M1.HpyAVI is a DNA adenine MTase that belongs to the type II R-M system. M1.HpyAVI encoded by ORF hp0050 is an N6-adenine methyltransferase belonging to the β-class MTase. It has been reported recently that this enzyme recognizes the sequence of 5′-GAGG-3′, 5′-GGAG-3′ or 5′-GAAG-3′ and methylates adenines in these sequences. The structural basis and the catalytic mechanism underlying such a distinct activity are not well understood due to the lack of an available 3D structure of this enzyme.Here, we report the crystal structure of M1.HpyAVI from H. pylori 26695, which is the first determined N6-adenine MTase structure in H. pylori.

The cofactor-free and AdoMet-bound proteins were crystallized at different conditions. Both structures were determined by means of molecular replacement, and refined to 3.0 Å and 3.1 Å, respectively. Four and eight protein monomers resided in the asymmetric units of the two crystal structures. The two structures are very similar to each other and could be well overlaid with an RMSD of 0.76 Å on 191 Cα atoms. The catalytic motif DPPY lies in a loop connecting αD and β4, and the cofactor AdoMet binds in a neighboring cavity. The cofactor binding pocket of M1.HpyAVI is surrounded by residues 7-9, 29-31, 165-167, 216-218 and 221, which are conserved among most of DNA MTases. A hydrogen bond between D29 in the catalytic motif DPPY and the amino group of bound AdoMet is preserved as other MTase structures. Residues D8 and A9 from hydrogen-bonds with N6 and N1 of the purine ring, respectively, and E216 also locates at hydrogen bonding distance with O2′ and O3′ of the ribose. In addition, H168, T200 and S198 contact the terminal carboxyl of AdoMet. The phenyl ring of F195 forms a perpendicular π-stacking interaction with the purine ring of AdoMet, which stabilizes the orientation of AdoMet bound in the pocket of M1.HpyAVI.

>MIQIYHADAFEIIKDFYQQNLKVDAIITDPPYNISVKNNFPTLKSAKRQGIDFGEWDKNFKLLEWIARYAPLVNPNGCMVIFCSYRFISYIADFLEENGFVVKDFIQWVKNNPMPRNIHRRYVQDTEFALWAVKKKAKWVFNKPKNEKYLRPLILKSPVVSGLEKTKHPTQKSLALMEKIISIHTNPNDIVLDPFMGSGTTGLACKNLERNFIGIESEKEYFQTAKKRLNLF[8x]>[6x]AVSVALGQTVRITCQGDSLRSYS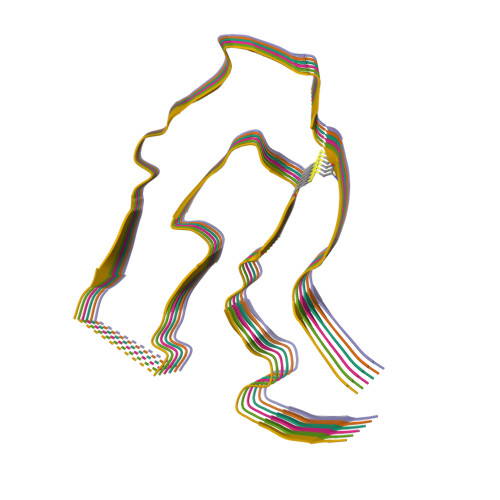ASWYQQKPGQAPVLVIFRNTASLTITGAQAEDEADYYCNSRDSSANHQVFGGGTKLTV> SSPPVVDTVHGKVLGKFVSLEGFAQPVAIFLGIPFAKPPLGPLRFTPPQPAEPWSFVKNATSYPPMCTQDPKAGQLLSELFTNRKENIPLKLSEDCLYLNIYTPADLTKKNRLPVMVWIHGGGLMVGAASTYDGLALAAHENVVVVTIQYRLGIWGFFSTGDEHSRGNWGHLDQVAALRWVQDNIASFGGNPGSVTIFGEAAGGESVSVLVLSPLAKNLFHRAISESGVALTSVLVKKGDVKPLAEQIAITAGCKTTTSAVMVHCLRQKTEEELLETTLKMKFLSLDLQGDPRESQPLLGTVIDGMLLLKTPEELQAERNFHTVPYMVGINKQEFGWLIPMLMSYPLSEGQLDQKTAMSLLWKSYPLVCIAKELIPEATEKYLGGTDDTVKKKDLFLDLIADVMFGVPSVIVARNHRDAGAPTYMYEFQYRPSFSSDMKPKTVIGDHGDELFSVFGAPFLKEGASEEEIRLSKMVMKFWANFARNGNPNGEGLPHWPEYNQKEGYLQIGANTQAAQKLKDKEVAFWTNLFAK

Carboxylesterases are a family of enzymes that act on a variety of both exogenous (e.g. cocaine, heroin) and endogenous (e.g. acyl-CoA esters) substrates. They are defined by their ability to hydrolyze ester, amide, or thioester bonds to their corresponding alcohol, amine or thiol and free acid in a diverse range of chemically distinct compounds. Carboxylesterases comprise three distinct domains; a central domain containing the catalytic triad (S221, H467 and E354), a regulatory domain (RD) and an α/β domain. The active site occupies a 10-15Å deep hydrophobic pocket at the interface of the three domains with all three catalytic residues arranged such that a proton transfer chain can be established.

The structure-function relationship of this aglycosylated hCES1 was explored alongside the wild type enzyme and a catalytically inactive mutant (S221A). Here, recombinant hCES1 enzymes were produced in HEK293 cells using either transient expression (hCES1 N79Q) or from stable cell lines (hCES1 and S221A). The HEK Gnt1-/- mutant cell line in which N-glycosylation is restricted to GlcNAc2Man5 was used for generating stable cell lines. In all three structures, the asymmetric unit contained one monomer of hCES1, containing, two disulphide bridges were present, C87- C116 and C274—C285 as seen in other hCES1 structures. In the crystal structure of hCES1 and hCES1 S221A, an N-acetylglucosamine adduct was observed attached to the side chain of residue N79. Space group symmetry was used to generate the biological trimer that is seen in solution. Superposition of the monomeric structures showed no differences between the glycosylated and aglycosylated hCES1. The orientation of the side-chains of the catalytic triad (S221, E354, H467) in bound and unbound enzymes was also identical showing that the enzyme is pre-disposed for substrate binding.>VQIGPVTDLHIVNADIVPDGFVRPAVNAGGTFPGPVIAGNVGDNFQIVTFNQLIECSMLVDTSIHWHGEFQKGTNWADGPAFITQCPIIVGNSFSYNFNVPGMAGTYWYHSHLTTQYCDGLRGPFVVYDPNDPDANLYDVDDDTTIITLADWYHVLAKEMGAGGAITADSTLIDGLGRTHVNVAAVPLSVITVEVGKRYRMRLVSISCDPNYDFSIDGHDMTIIETDGVDSQELTVDEIQIFAAQRYSFVLNANQPVGNYWIRANPNSGGEGFDGGINSAILRYDGATTADPVTVASTVHTKCLIETDLHPLSRNGVPGNPHQGGADCNLNLSLGFACGNFVINGVSFTPPTVPVLLQICSGANTAADLLPSGSVISLPSNSTIEIALPAGAAGGPHPFHLHGHDFAVSESASNSTSNYDDPIWRDVVSIGGVGDNVTIRFCTDNPGPWFLHCHIDWHLDAGFAIVFAEDIPNTASA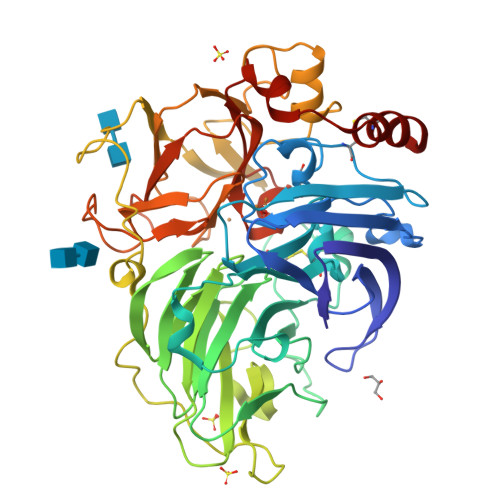NPVPEAWSNLCPSYDSAH[3x]>[2x]SMAIRVADLLQHITQMKRGQGYGFKEEYEALPEGQTASWDTAKEDENRNKNRYGNIISYDHSRVRLLVLDGDPHSDYINANYIDGYHRPRHYIATQGPMQETVKDFWRMIWQENSASIVMVTNLVEVGRVKCVRYWPDDTEVYGDIKVTLIETEPLAEYVIRTFTVQKKGYHEIRELRLFHFTSWPDHGVPCYATGLLGFVRQVKFLNPPEAGPIVVHCSAGAGRTGCFIAIDTMLDMAENEGVVDIFNCVRELRAQRVNLVQTEEQYVFVHDAILEACLCGNTAI

Protein tyrosine phosphatases (PTPs) play a critical role in regulating cellular functions by selectively dephosphorylating their substrates. The ∼280 residue PTP catalytic domain consists of an α/β structure, and biochemical and structural studies have led to a detailed understanding of the catalytic mechanism (Barford et al., 1994; Zhang, 2002). Key features of the domain include the PTP signature motif, the mobile Trp-Pro-Asp “WPD” loop that in the closed conformation positions the conserved and catalytically important aspartate residue, and the phosphotyrosine recognition loop. Here we report the crystal structures of 22 PTP domains, including two tandem-domain RPTP structures and a detailed structural comparison of this protein family.

In the fourth category, both the gateway and secondary pocket are blocked and the inaccessible binding cavity harbors an aromatic residue or a proline in position of Arg24. The second-site loop assumes a twisted conformation in these phosphatases. This architecture is present in the subgroups NT5 (PTPH1, MEG1), NT6 (PTPD1, PTPD2), R1 (CD45), R2B (RPTPμ, RPTPκ, RPTPρ), and R4 (RPTPα, RPTPɛ). In contrast R1 group members (e.g., CD45) and R2B group had a more than two orders of magnitude lower enzymatic activity, suggesting that enhancement of activity by tight association with substrates in signaling complexes may be important for efficient signaling.>[6x]GS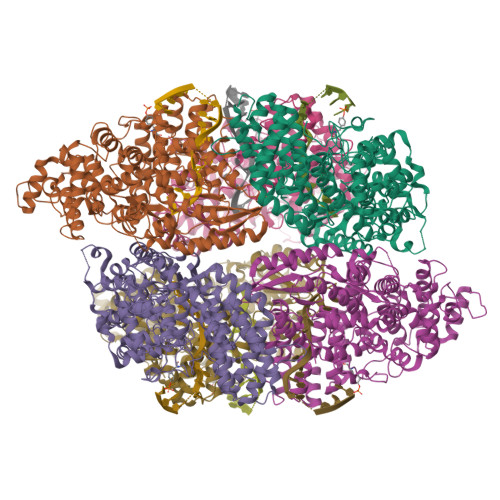MKKEFTELYDFIFDPIFLVRYGYYDRSIKNKKMNTAKVELDNEYGKSDSFYFKVFNMESFADYLRSHDLKTHFNGKKPLSTDPVYFNIPKNIEARRQYKMPNLYSYMALNYYICDNKKEFIEVFIDNKFSTSKFFNQLNFDYPKTQEITQTLLYGGIKKLHLDLSNFYHTLYTHSIPWMIDGKSASKQNRKKGFSNTLDTLITACQYDETHGIPTGNLLSRIITELYMCHFDKQMEYKKFVYSRYVDDFIFPFTFENEKQEFLNEFNLICRENNLIINDNKTKVDNFPFVDKSSKSDIFSFFENITSTNSNDKWIKEISNFIDYCVNEEHLGNKGAIKCIFPVITNTLKQKKVDTKNIDNIFSKRNMVTNFNVFEKILDLSLKDSRLTNKFLTFFENINEFGFSSLSASNIVKKYFSNNSKGLKEKIDHYRKNNFNQELYQILLYMVVFEIDDLLNQEELLNLIDLNIDDYSLILGTILYLKNSSYKLEKLLKKIDQLFINTHANYDVKTSRMAEKLWLFRYFFYFLNCKNIFSQKEINSYCQSQNYNSGQNGYQTELNWNYIKGQGKDLRANNFFNELIVKEVWLISCGENEDFKYLN> MSCMDLDVITTVVKIEGKLRNETLLRVGKGKTQDFAEATDNPIIKYRDRPLIPGSSLKGAFRSLVESYTKSLNDSKYYVCDLDDNSCVSCEEKKKDNGIVEGRYCIPCILFGFKDLASRVYILDAIAEKYSISQRTMVAINRVF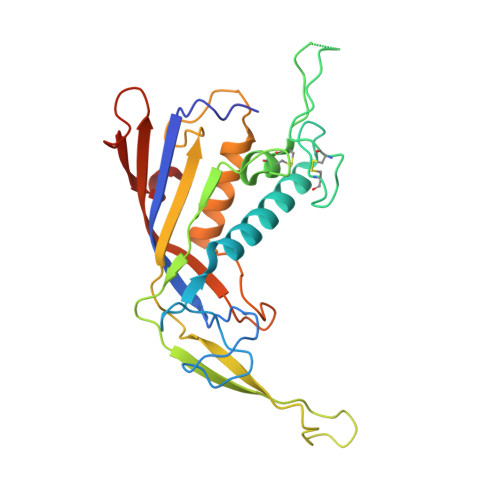GGQMPGHLYTLDYVDPGSEFSFMMMIYNLNLIEGEKDWKAKSVEALKFLLATLVREGIFVGARKSVGYGLIKLVDAKVSLYKAPDHLVSPVIVKKLEEVIGTNG> SEFENPLKRLLVPGEEWEFEVTAFYRGRQVFQQTISCPEGLRLVGSEV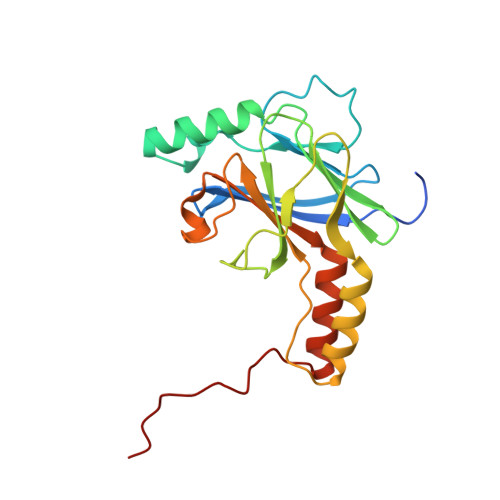GDRTLPGWPVTLPDPGMSLTDRGVMSYVRHVLSCLGGGLALWRAGQWLWAQRLGHCHTYWAVSEELLPNSGHGPDGEVPKDKEGGVFDLGPFIVDLITFTEGSGRSPRYALWFCVGESWPQDQPWTKRLVMVKVVPTCLRALVEMARVGGASELENTVDLHIENS N'-[4-[[(2S,4R)-4-[3-[(C-thiophen-2-ylcarbonimidoyl)amino]phenoxy]pyrrolidin-2-yl]methoxy]phenyl]thiophene-2-carboximidamide 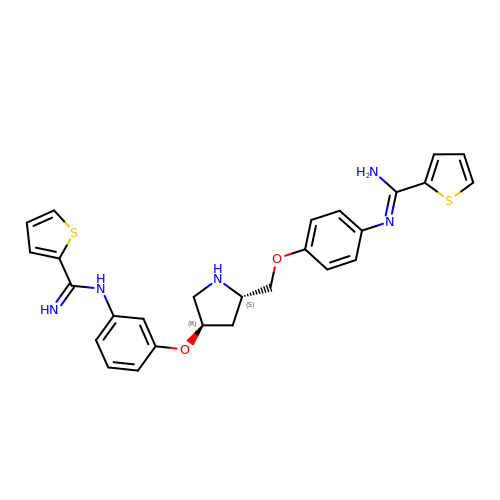| C27 H27 N5 O2 S2 | MVLJJSCAHWVTFO-NZQKXSOJSA-N> NSLRACGPALMDMLRVACPN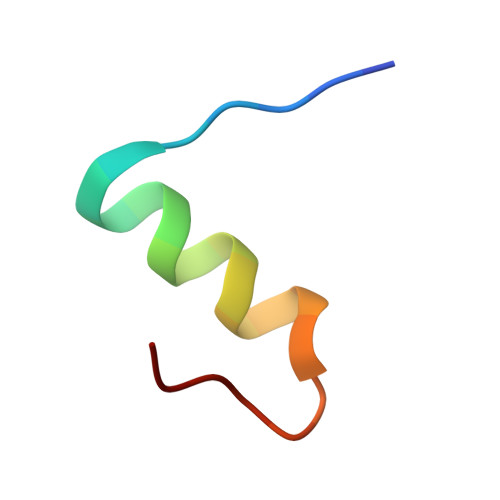GFNS> GPLGSLKKQYIFQLSSLNPQER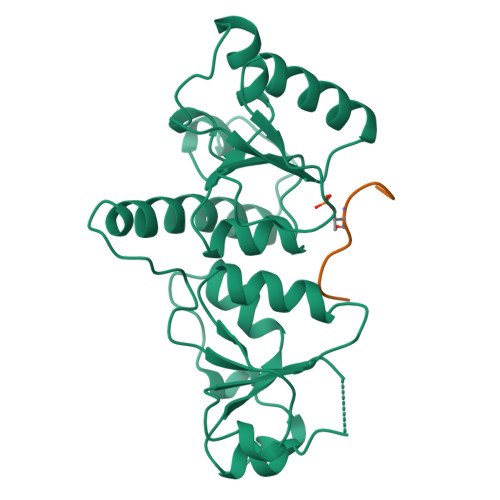IDYCHLIEKLGGLVIEKQCFDPTCTHIVVGHPLRNEKYLASVAAGKWVLHRSYLEACRTAGHFVQEEDYEWGSSSILDVLTGINVQQRRLALAAMRWRKKIQQRQESGIVEGAFSGWKVILHVDQSREAGFKRLLQSGGAKVLPGHSVPLFKEATHLFSDLNKLKPDDSGVNIAEAAAQNVYCLRTEYIADYLMQESPPHVENYCLPEAISFI;> SIYFTPELYD5-amino-D-isoleucine | C6 H14 N2 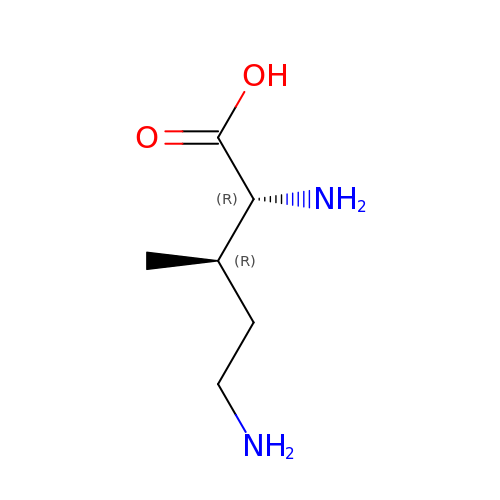O2 | HYUPFEBCCJWDJX-RFZPGFLSSA-N>QQSKPEDLLKLRQGLMQTL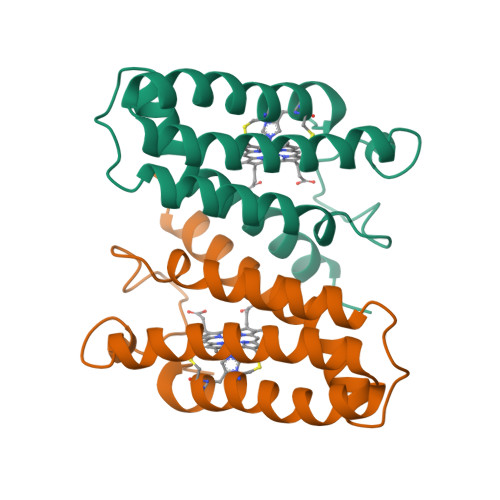KSQWVPIAGFAAGKADLPADAAQRAENMAMVAKLAPIGWAKGTEALPNGETKPEAFGSKSAEFLEGWKALATESTKLAAAAKAGPDALKAQAAATGKVCKACHEEFKQD[2x]> 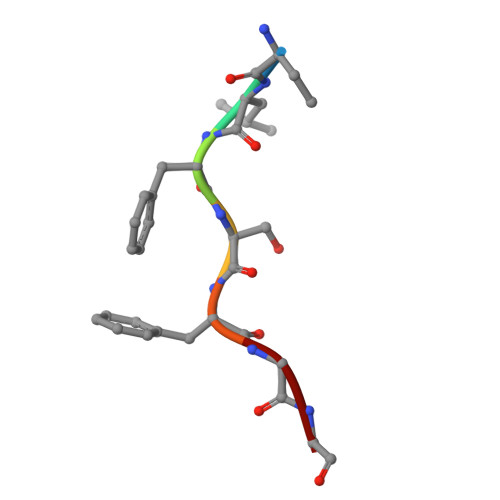KLFSFGG>[4x]MAGDTTITIV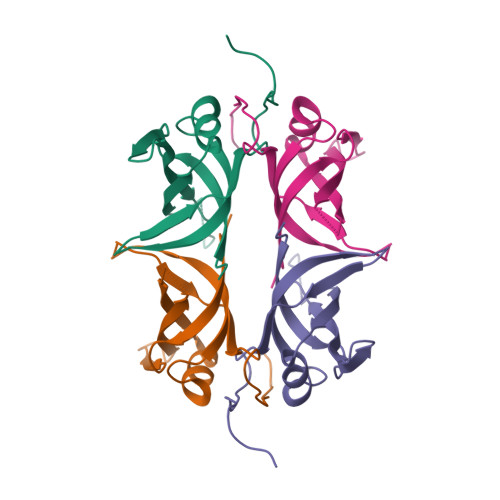GNLTADPELRFTPSGAAVANFTVASTPRIYDRQTGEWKDGEALFLRCNIWREAAENVAESLTRGARVIVSGRLKQRSFETREGEKRTVIEVEVDEIGPSLRYATAKVNKASRSGGFGSGSRPAPAQTSSASGDDPWGSAPASGSFGGGDDEPPF>[5x]AQDMVSPPPPIADEPLTVNTGIYLIECYSLDDKAETFKVNAFLSLSWKDRRLAFDPVRSGVRVKTYEPEAIWIPEIRFVNVENARDADVV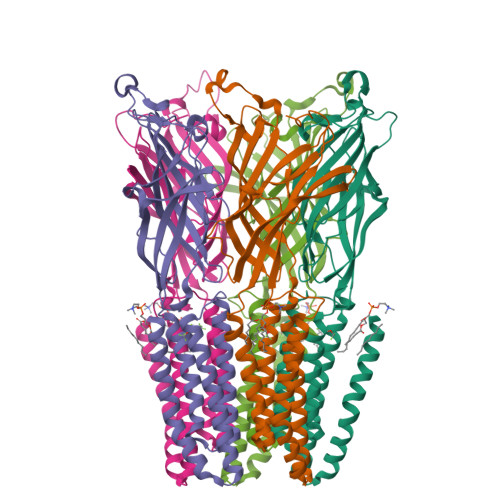DISVSPDGTVQYLERFSARVLSPLDFRRYPFDSQTLHIYLIVRSVDTRNIVLAVDLEKVGKNDDVFLTGWDIESFTAVVKPANFALEDRLESKLDYQLRISRQYFSYIPNIILPMLFILFISWTAFWSTSYEANVTLVVSTLIAHIAFNILVETNLPKTPYMTYTGAIIFMIYLFYFVAVIEVTVQHYLKVESQPARAASITRASRIAFPVVFLLANIILAFLFFGFG> MNKQIFVLYFNIFLIFLGIGLVIPVLPVYLKDLGLTGSDLGLLVAAFALSQMIISPFGGTLADKLGKKLIICIGLILFSVSEFMFAVGHNFSVLMLSRVIGGMSAGMVMPGVTGLIADISPSHQKAKNFGYMSAIINSGFILGPGIGGFMAEVSHRMPFYFAGALGILAFIMSIVLIHDPKKSTTSGFQKLEPQLLTKINWKVFITPVILTLVLSFGLSAFETLYSLYTADKVNYSPKDISIAITGGGIFGALFQIYFFDKFMKYFSELTFIAWSLLYSVVVLILLVFANDYWSIMLISFVVFIGFDMIRPAITNYFSNIAGERQGFAGGLNSTFTSMGNFIGPLIAGALFDVHIEAPIYMAIGVSLAGVVIVLIEKQHRAKLKEQNMENLYFQGKLGPEQKLISEE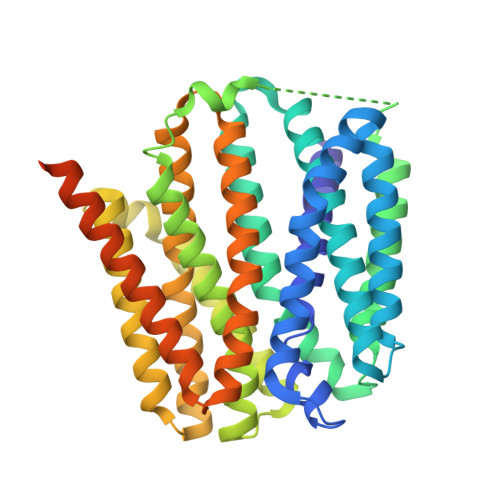DLNSAVDHHHHHHHHHH>MEAFEISDFKEHAKKKSMWAGALNKVTISGLMGVFTEDEDLMALPIHRDHCPALLKIFDELIVNATDHERACHSKTKKVTYIKISFDKGVFSCENDGPGIPIAKHEQASLIAKRDVYVPEVASCFFLAGTNINKAKDCIKGGTNGVGLKLAMVHSQWAILTTADGAQKYVQQINQRLDIIEPPTITPSREMFTRIELMPVYQELGYAEPLSETEQADLSAWIYLRACQCAAYVGKGTTIYYNDKPCRTGSVMALAKMYTLLSAPNSTIHTATIKADAKPYSLHPLQVAAVVSPKFKKFEHVSIINGVNCVKGEHVTFLKKTINEMVIKKFQQTIKDKNRKTTLRDSCSNIFVVIVGSIPGIEWTGQRKDELSIAENVFKTHYSIPSSFLTSMTRSIVDILLQSISKKDNHKQVDVDKYTRARNAGGKRAQDCMLLAAEGDSALSLLRTGLTLGKSNPSGPSFDFCGMISLGGVIMNACKKVTNITTDSGETIMVRNEQLTNNKVLQGIVQVLGLDFNCHYKTQEERAKLRYGCIVACVDQDLDGCGKILGLLLAYFHLFWPQLIIHGFVKRLLTPLIRVYEKGKTMPVEFYYEQEFDAWAKKQTSLVNHTVKYYKGLAAHDTHEVKSMFKHFDNMVYTFTLDDSAKELFHIYFGGESELRKRELCTGVVPLTETQTQSIHSVRRIPCSLHLQVDTKAYKLDAIERQIPNFLDGMTRARRKILAGGVKCFASNNRERKVFQFGGYVADHMFYHHGDMSLNTSIIKAAQYYPGSSHLYPVFIGIGSFGSRHLGGKDAGSPRYISVQLASEFIKTMFPAEDSWLLPYVFEDGQRAEPEYYVPVLPLAIMEYGANPSEGWKYTTWARQLEDILALVRAYVDKDNPKHEL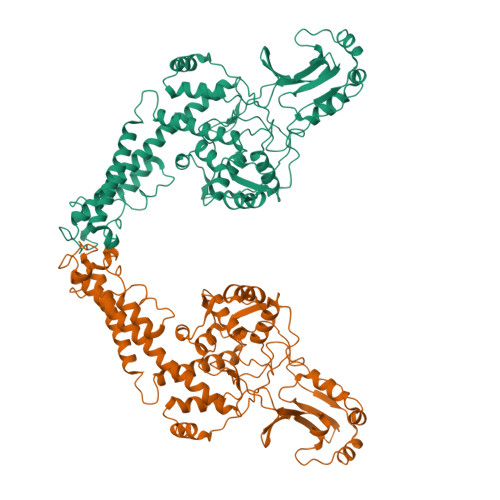LHYAIKHKITILPLRPSNYNFKGHLKRFGQYYYSYGTYDISEQRNIITITELPLRVPTVAYIESIKKSSNRMTFIEEIIDYSSSETIEILVKLKPNSLNRIVEEFKETEEQDSIENFLRLRNCLHSHLNFVKPKGGIIEFNSYYEILYAWLPYRRELYQKRLMREHAVLKLRIIMETAIVRYINESAELNLSHYEDEKEASRILSEHGFPPLNHTLIISPEFASIEELNQKALQGCYTYILSLQARELLIAAKTRRVEKIKKMQARLDKVEQLLQESPFPGASVWLEEIDAVEKAIIKGRNTQWKFHHHHHH[2x]> LRSRRKPSSRIGRRPSTTQDRISTVGIELFTEQGFDATSVDEVAEASGIARRTLFRYFPSKNAIPWGD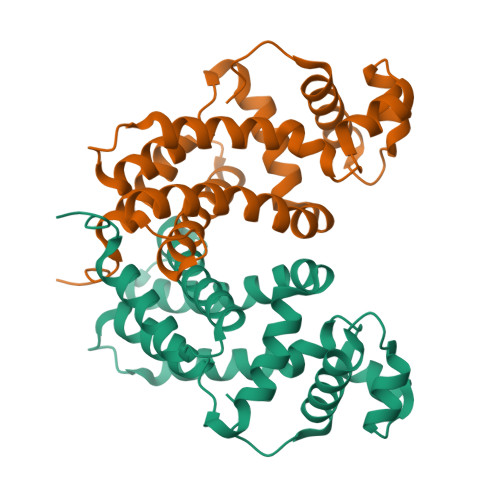FDAHLAEMRAQLAAQPDDIPIVDGLTAALLQFNAFPASEEINHRKRMGLILRVPALQAYSVVMYEGWRNVIAEYVASRLGTSPTDHVPRTVGYLLLGVAMSAYEQWLDDDSLELNELLASGMQSLYDGLSSLGEPDTRT>VSIKKSSGLNFDNTAIAINAGKGLEFDTNTSESPDINPIKTKIGSGIDYNENGAMITKLGAGLSFDNSGAITIGNKNDDKLTLWTTPDPSPNCRIHSDNDCKFTLVLTKCGSQVLAT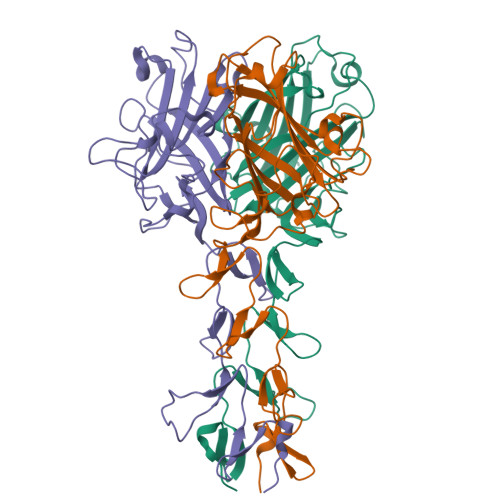VAALAVSGDLSSMTGTVASVSIFLRFDQNGVLMENSSLKKHYWNFRNGNSTNANPYTNAVGFMPNLLAYPKTQSQTAKNNIVSQVYLHGDKTKPMILTITLNGTSESTETSEVSTYSMSFTWSWESGKYTTETFATNSYTFSYIAQE[6x]>[2x]MVNRIQNPILPGFHPDPSIVRVGDDYYIATSTFEWFPGVRIHHSRDLKHWRFVSSPLTRTSQLDMKGNMNSGGIWAPCLSYHDGTFYLIYTDVKQWHGAFKDAHNYLVTAQNIEGPWSDPIYLNSSGFDPSLFHDDDGRKWLVNMIWDYRKGNHPFAGIILQEYSEAEQKLVGPVKNIYKGTDIQLTEGPHLYKKDGYYYLLVAEGGTEYEHAATLARSQSIDGPYETDPSYPLVTSTGQPELALQKAGHGSLVETQNGEWYLAHLCGRPLKGKYCTLGRETAIQKVNWTEDGWLRIEDGGNHPLREVTAPDLPEHPFEKEPELDDFDAPQLHHQWNTLRIPADPSWCSLEERPGHLRLRGMESLTSVHSQSLVARRQQSFHCEVETKLEYQPESFQHMAGLVIYYDTEDHVYLHV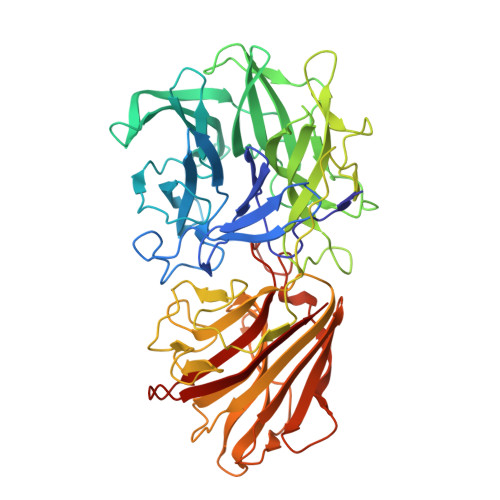TWHEEKGKCLQIIQTKGGNYDELLASPIPLAEEKAVYLKGRIHRETMHLYFKQEGEAEWQPVGPTIDVTHMSDDSAKQVRFTGTFVGMATQDLSGTKKPADFDYFRYKELDQ> GHMK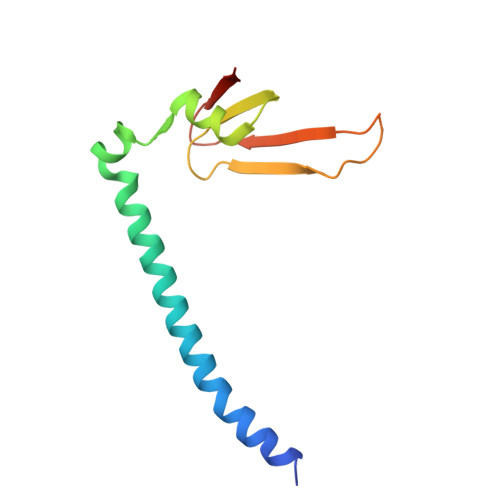EVIDRLRYLKAEIEDLELKERELDQQKLWLQQSIKNVMDDSINNRFSYVTHEDICNCFNGDTLLAIQAPSGTQLEVPIPEMGQNGQKKYQINLKSHSGPIHVLLINKE>MDYNLALDKAIQKLHDEGRYRTFIDIEREKGAFPKAQWNRPDGGKQDITVWCGNDYLGMGQHPVVLAAMHEALEAVGAGSGGTRNISGTTAYHRRLEAEIAGLHQKEAALVFSSAYNANDATLSTLRVLFPGLIIYSDSLNHASMIEGIKRNAGPKRIFRHNDVAHLRELIAADDPAAPKLIAFESVYSMDGDFGPIKEICDIAEEFGALTYIDEVHAVGMYGPRGAGVAERDGLMHRIDIFNGTLAKAYGVFGGYIAASARMVDAVRSYAPGFIFSTSLPPAIAAGAQASIAFLKTAEGQKLRDAQQMHAKVLKMRLKALGMPIIDHGSHIVPVVIGDPVHT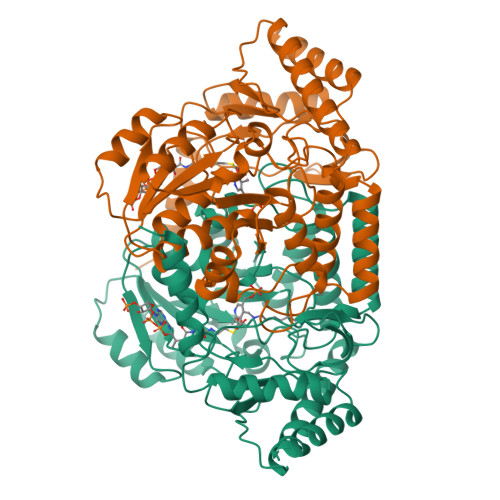KAVSDMLLSDYGVYVQPINFPTVPRGTERLRFTPSPVHDLKQIDGLVHAMDLLWARCA[4x]>[2x]GTACG;>[2x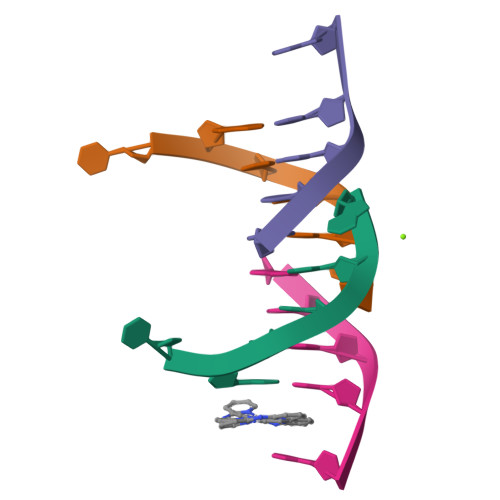]CGTACG>[4x]KGPNLTEISKKITESNAVVLAVKEVETLLTSIDELAKAIGKK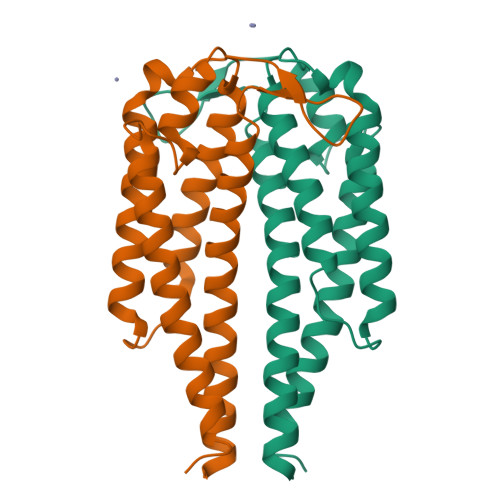IKSDVSLDNEADHNGSLMSGAYLISTLITKKISAIKDSGELKAEIEKAKKCSEEFTAKLKGEHTDLGKEGVTDDNAKKAILKTNNDKTKGADELEKLFESVKNLSKAAKEMLTNSVKELTSP> MREKRGNRKALDPVGEDGVTGKDGKGFFACYLLTSLSPRHKGQTYIGFTVNPRRRIRQHNGEITSGAWRTKKKRPW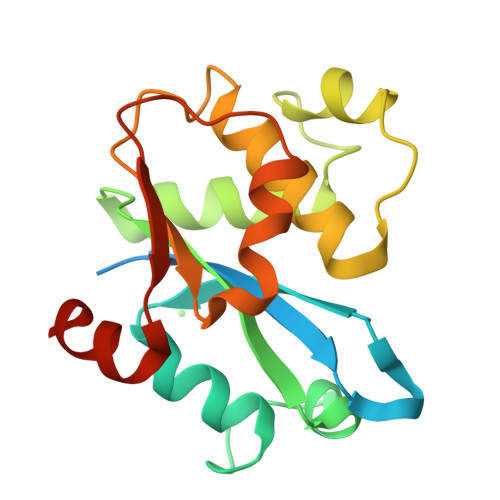EMVLCIYGFPTNVSALQFEWAWQHPRESVAVREAAAAFKSFSGVASKIKLVYTMLNLPAWNSLNLTVNYFSSKYAHHGGKSPSLPLHMKVQVCAMEDLQYFTKVDDS> NTAVADYQKAKAEFPQKQEQYNKDFEKYQSDVKEYEAQKAAYEQYKKEVAQGLASGR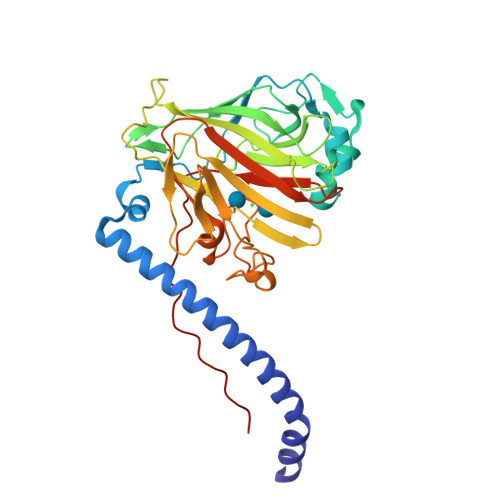VEKAQGLVFINEPEAKLSIEGVNQYLTKEARQKHATEDILQQYNTDNYTASDFTQANPYDPKEDTWFKMKVGDQISVTYDNIVNSKYNDKKISKVKINYTLNSSTNNEGSALVNLFHDPTKTIFIGAQTSNAGRNDKISVTMQIIFYDENGNEIDLSGNNAIMSLSSLNHWTTKYGDHVEKVNLGDNEFVKIPGSSVDLHGNEIYSAKDNQYKANGATFNGDGADGWDAVNADGTPRAATAYYGAGAMTYKGEPFTFTVGGNDQNLPTTIWFATNSAVAVPKDPGAKPTPPEKPELK>GAMGSNEYVEEQEAENSSKPDDSKIDEHTIGHVFHAMGVVHSKKDRKSLGKNIKVFYFSEEDGHFQTIPSKENAKLIVYFYDNVYAGEAPISISGKEAFIFVGITPD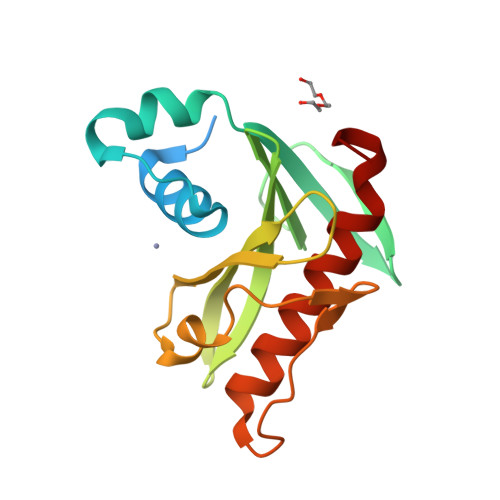FKKIINSNLHGAKSDLIGTFKDLNIKNSKLEITVDENNSDAKTFLESVNYIIDGVEKISPMLTN[2x]> SRHSEKIAIRDFQVGD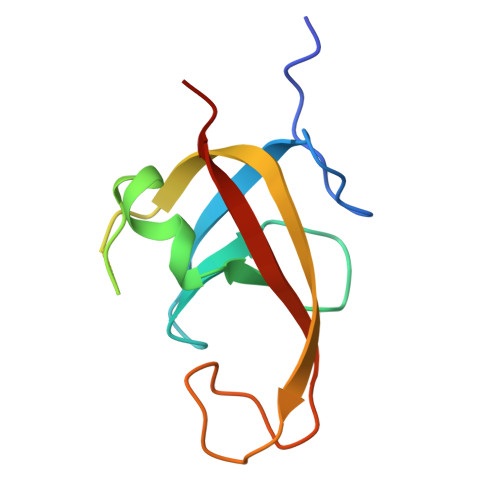LVLIILDERHDNYVLFTVSPTLYFLHSESLPALDLKPGEGASGASRRPWVLGKVMEKEYCQAKKAQNRFKVPLGTKFYRVKAVSWNKKV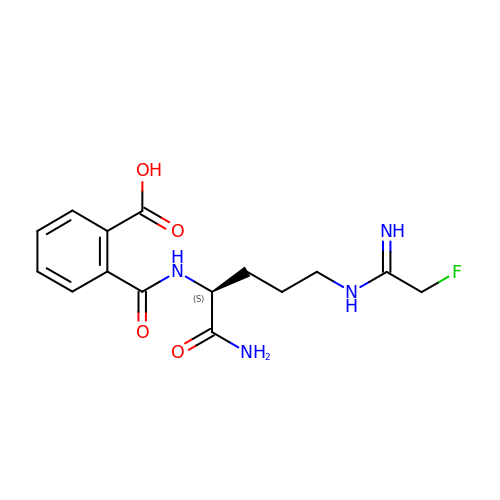2-{[(2S)-1-amino-5-{[(1Z)-2-fluoroethanimidoyl]amino}-1-oxopentan-2-yl]carbamoyl}benzoic acid | C15 H19 F N4 O4 | HBEIARVCIYYMOR-NSHDSACASA-N TETRACYCLINE 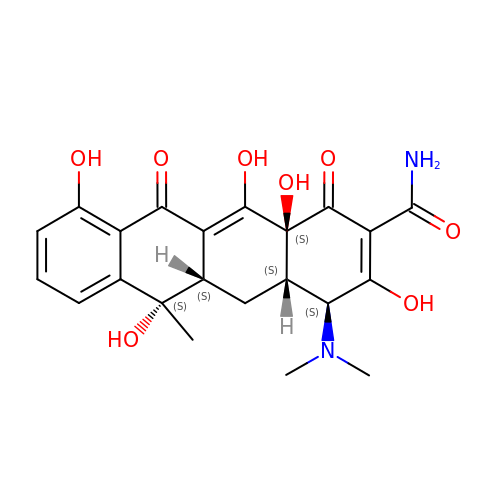| C22 H24 N2 O8 | OFVLGDICTFRJMM-WESIUVDSSA-N> GRC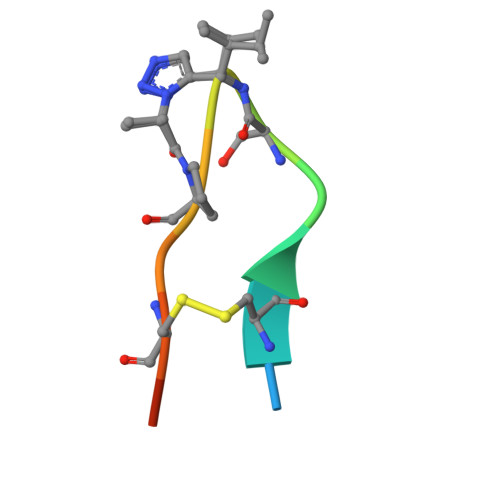TKSXPICFPD5-[AMINO(IMINO)METHYL]-2-[({[6-[3-AMINO-5-({[(1R)-1-METHYLPROPYL]AMINO}CARBONYL)PHENYL]-3-(ISOPROPYLAMINO)-2-OXOPYRAZIN-1(2H)-YL]ACETYL}AMINO)METHYL]-N-PYRIDIN-4-YLBENZAMIDE 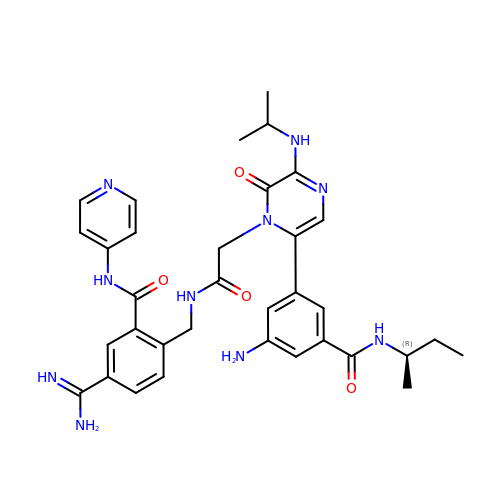| C34 H40 N10 O4 | HLQIVSDFLBJBKY-HXUWFJFHSA-N Proteins of the RRNPPA family are the most frequent pheromone receptors in Bacillota and use small secreted oligopeptides as pheromones. While most members of the RRNPPA family act as transcriptional factors through DNA binding, Rap receptors are specialized members that exhibit the capability to develop their function by interaction with specific protein targets. Binding of the pheromone produced from the propeptide, which is named Phr in this RRNPPA subfamily, induces Rap receptor inhibition. Our results reveal that distinct maturation processes generate multiple mature pheromones, which bind to receptors with varying affinities but produce identical structural and biological responses.

In addition to the 2 putative pheromones RRGHTA and SRGHTS, we included in the analysis an extended (RRGHTAS) and a shorter (RGHTS) version of the internal and C-terminal putative pheromones, respectively, that could represent alternative forms of their maturation. Rap3T shows 4 times lower affinity (EC50 20,75 nM) for the putative Phr3T C-terminal canonical pheromone (SRGHTS) and more than 10 times lower affinity (EC50 69,75 nM) for the possible maturation variant of this peptide with one less amino acid. To molecularly assess the differences in affinity and stabilization for the alternative peptides analyzed we solved the structures for Rap3T in complex with RRGHTAS, SRGHTS, and RGHTS. Meanwhile complexes with RRGHTAS and RGHTS peptides exhibited P21 space group and a Rap dimer in the asymmetric unit. Remarkably, these structures exhibited nearly identical conformations as confirmed by the low differences in the superimposition of their Cα atoms for either individual monomers or the complete dimers (RMSD 0.36–0.50), dispelling the notion of peptides eliciting divergent conformational shifts. Comparison of complexes with RRGHTA and SRGHTS peptides showed that the sidechain of Arg in position 1 for RRGHTA mediates a network of salt-bridges with D264 and D335 plus hydrophobic interactions with M304 meanwhile the Ser in this position for SRGHTS only makes a hydrogen bound with Y225. These differences in interactions for position 1 may explain the lower stabilization seen in thermal shift assays and the higher EC50 value from thermophoresis assays for SRGHTS. Accordingly, the complex with the shorter peptide (RGHTS) showed that this position is empty, explaining why this peptide shows the lowest affinity for the receptor.

>MLEQMISSSKVGVKINEWYKYIRLFSVPDSEILKAEVEEEIRHMKEDHDLLLYYSLMCFRHQLMLDYLEPKTLNEERPKISDLLEKIESSQTDLKGILEYYFNFFRGMYEFEQYEYLNAISFYKQAERKLSLVADEIERAEFHYKVAEIYYHMKQTHMSMHHIVQAIDSYKAHENYTVRVIQCSFVIGLNYLDMDYPEKAIPHFKNALDKAREIDMSRLIGSSLYNLGLCSFAEEAYEKASEYFKEGIRVYQDNGYEHSNRILDILLMLTKTTFKMRNHSEGISWCAHGLSLSKNLNDEIMAKMFEFIHALYVDNDNEKLNSILNYLELKSMLSDVEDLASDAAKYYNEKEDHKVAVAYYEKVLYARKQIQRGDCLYET[2x];>[2x]RGHTS> 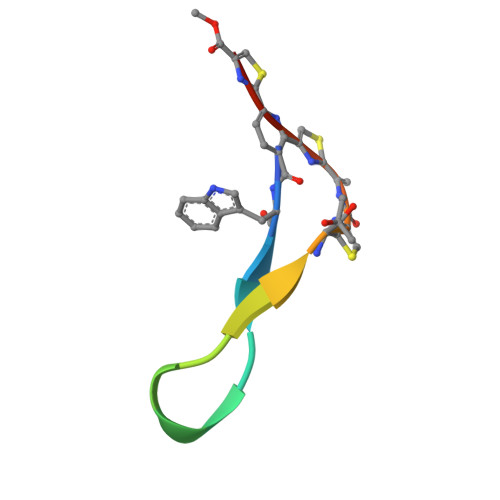SWTIRTRGRIATCSCSCX tert-butyl 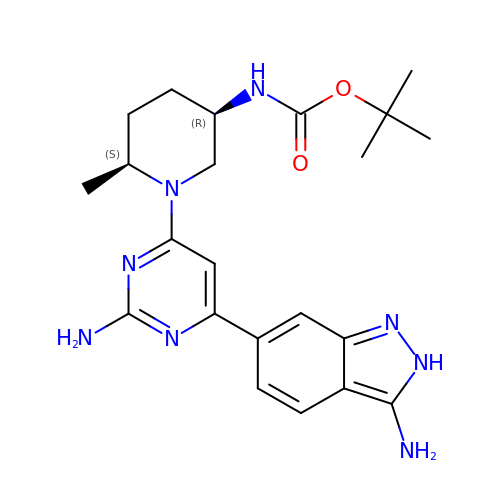{(3R,6S)-1-[2-amino-6-(3-amino-2H-indazol-6-yl)pyrimidin-4-yl]-6-methylpiperidin-3-yl}carbamate | C22 H30 N8 O2 | GAMJJHMLLXIWRZ-GXTWGEPZSA-N We have focused our work on the iron(II)/α-KetoAcid-dependent Oxygenases (αKAOs), a mechanistically diverse superfamily of enzymes that use dioxygen as the oxidant to catalyze several reactions via C-H bond activation, mostly hydroxylation. These enzymes operate with three substrates, dioxygen, α-ketoglutarate (α-KG) and a primary substrate. One of these, KDO1, catalyzes the formation of (3S)-3-hydroxy-L-lysine, while five others, KDO2 to KDO6, promote the formation of (4R)-4-hydroxy-L-lysine. We based our analysis on the structures that we solved by X-ray crystallography of two of the regiodivergent αKAOs active towards L-lysine, namely KDO1 from Catenulispora acidiphila, that catalyzes the C-3 hydroxylation, and KDO5, from Flavobacterium sp., that catalyzes the C-4 hydroxylation.

The structure of the apo form of KDO1 was determined without iron in the active site, lost during purification, while KDO5 retained the iron throughout. While a ferrous ion is present in the KDO5 apo structure, it is not the case in KDO1 apo as the metal is lost during the purification from the KDO1 preparation used to grow the crystals. After crystal soaking with FeSO4 the two His residues (178 and 314) and Glu180 in the KDO1 active site recapture an iron. For KDO1, the lid is well defined both in the apo and complexed forms, but the adjacent loop, from Ala160 to Ser171 (not in the logo except for P5 and P6, respectively residues 167 and 168) undergoes large conformational changes. Among all CSL dioxygenases whose crystal structures have been reported so far, this is the first time such a loop motion is observed. Its motion seems to be induced by α-KG binding as this loop is closed in apo and complexed forms with products and lysine, but opened when α-KG is bound.

>[4x]MKNLSAYEVYESPKTSGESRTEAVSEAAFESDPEVSAILVLTSSEASTLERVADLVTAHALYAAHDFCAQAQLAAAELPSRVVARLQEFAWGDMNEGHLLIKGLPQVRSLPPTPTSNVHAVAATTPMSRYQALINECVGRMIAYEAEGHGHTFQDMVPSAMSAHSQTSLGSAVELELHTEQAFSPLRPDFVSLACLRGDPRALTYLFSARQLVATLTTQEIAMLREPMWTTTVDESFLAEGRTFLLGFERGPIPILSGADDDPFIVFDQDLMRGISAPAQELQQTVIRAYYAERVSHCLAPGEMLLIDNRRAVHGRSIFAPRFDGADRFLSRSFIVADGSRSRHARSSFGRVVSARFS5-methyl-7-(naphthalen-2-ylamino)-1H-[1,2,4]triazolo[1,5-a]pyrimidine-3,8-diium | C16 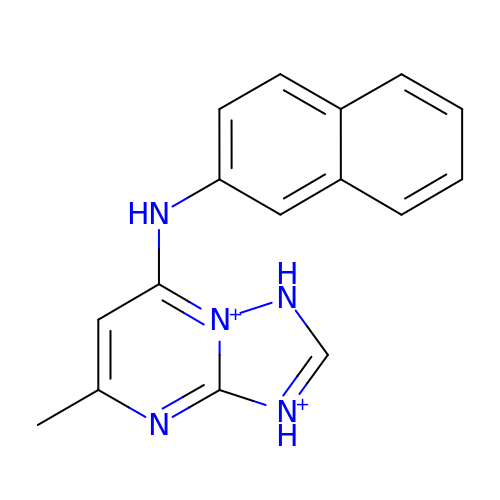H15 N5 | GNJXIZOPHGMAQW-UHFFFAOYSA-P>[2x]XSLSAKDKANVKAIWGKILPKSDEIGEQALSRMLVVYPQTKAYFSHWASVAPGSAPVKKHGITIMNQIDDCVGHMDDLFGFLTKLSELHATKLRVDPTNFK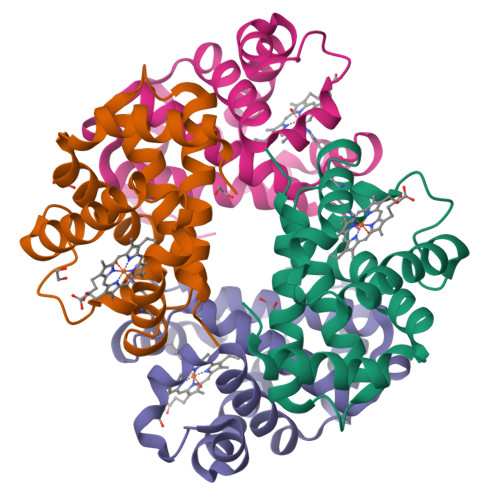ILAHNLIVVIAAYFPAEFTPEIHLSVDKFLQQLALALAEKYR;>[2x]VDWTDAERSAIVGLWGKISVDEIGPQALARLLIVSPWTQRHFSTFGNLSTPAAIMGNPAVAKHGKTVMHGLDRAVQNLDDIKNTYVTLSVMHSEKLFVDPDNFRLLADCITVCVAAKLGPAVFSADTQEAFQKFLAVVVSALGRQYH> LDFSKWKTRQPGEFRAPCPAMNSLANHGFIPRDGRNITVAMLVPVLQEVFHLSPELAQTISTLGLFTAQDPSKGVFTLDDLNRHNLFEHDASLSREDYYF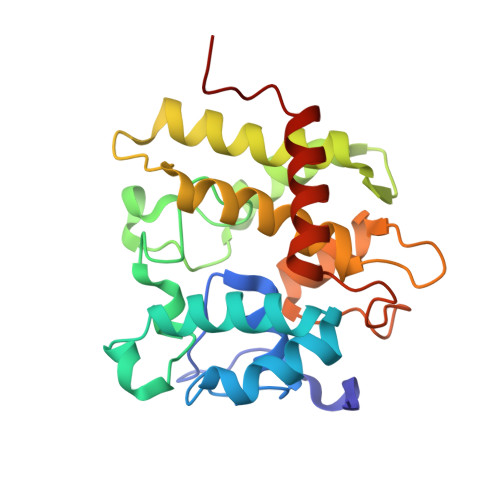HKDASTFRPEVFKKFMSHFKGKEYVTLEDAASARYAMVQESRKKNPTFTYTVQQRITSYGETIKYFRTIVEPATGKCPVAWIKILFEQERLPYNEGWRPPKAELSGFSMASDVLELALVTPEKLID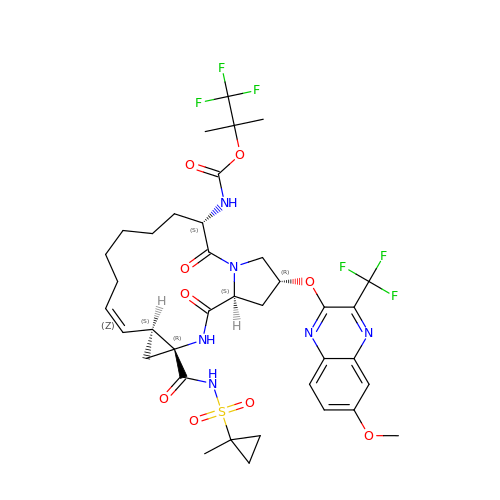1,1,1-trifluoro-2-methylpropan-2-yl [(2R,6S,12Z,13aS,14aR,16aS)-2-{[6-methoxy-3-(trifluoromethyl)quinoxalin-2-yl]oxy}-14a-{[(1-methylcyclopropyl)sulfonyl]carbamoyl}-5,16-dioxo-1,2,3,5,6,7,8,9,10,11,13a,14,14a,15,16,16a-hexadecahydrocyclopropa[e]pyrrolo[1,2-a][1,4]diazacyclopentadecin-6-yl]carbamate | C37 H44 F6 N6 O9 S | OJOOKWRLZOVJGU-SFBXLYIVSA-N> CEGPVHKSIPYVLQPEQIIPGVADYYATTVFDGFDFANLLVKTREGRPIKIENNTIAGAKFSANARIHASILGLYDSMRLKEPKLDGKNSSWSAVDLKIKSSLADAKAKGGQVVLLTNTLASPTTEKLIGEFIAKNPNAKHVVYDAVSSSDALDAFETVYGERALVDYDFSKASLIVSVGADFLGDWQGGGYDAGYAKGRIPQNGKMSRHFQFESNMTLSGAAADKRVPMTTADQKQALVQIYNIVVGASVPVSLDAKFKAEVVKAAQQLKAAGTKGILVSGIEDKNAQLLVLAINQALASEAFSTAGTRQIRKGSNAVVAQLIKDMNAGSVHTLIMSGVNPVYTLADSASFVSGLKKVKTSVAFSLKEDETAAVSTIAAAAPHYLESWGDVEITKGTYSLTQPTIRPIFDTKQFQDVLLSVNGTPGNFYDYLKANSGAIIAGSSWNKVLHDGIFVVGSAALAGGSYDFAGAASLLSKAKSSGELELVLYTKTGMGDGQHANNPWLQEFPDPITRVSWDNYVTVSNADAKKFNLSNEIVANGGLNGSYATITTADGNKLENVPVIVQPGQAVGTVGLAVGYGRKAALKEEMQVGINAYALYKNFNSVQSITLAKANGEHEFACVQGQKTLMGRGDIIKETTLEIFNTQDAKHWNEQPMVSLDHQEVEATTVDLWESFDRTTGHHFNLSIDLNACTGCGACVIACHAENNVPVVGKAEVRRSRDMHWLRIDRYYSSESTFEGDNERKEGIAGLSSSLSTFNEMEKPGDNPQVAFQPVMCQHCNHAPCETVCPVAATSHGRQGQNHMAYNRCVGTRYCANNCPYKVRRFNWFLYNKNSEFDY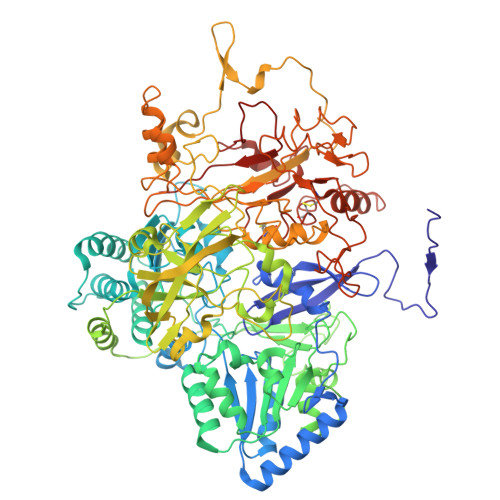HMNDDLGRMVLNPDVNVRSRGVMEKCSFCIQSTQAVILEAKRQGRVVGKDEFNNACACSAACSSGAMVFGDVNDKESEVAKLAESERMYHLLEHVGTKPNVFYHVKVRN>MKQYQMYVGGEWIDASNGQTEPVVSPINEEVLAYIQDADASDAERVLAVATTAQKEWAKQPARQRAEVLRKFAQLIRDNKQYLAELLVKEQGKLLKVALGEVEATSTFIEYACDWARQMDGDIVKSDNANEQIMIHKIPRGVVVAITAWNFPLALAGRKIGPALVAGNSIVVKPTSETPLATLELGYLAEQAGIPAGVLNIVTGGGRTLGNELVGHRMTNMVSMTGSTPAGQSIIRASANNMAHVQLELGGKAPFIVMEDADLEQAAAAALHSRFDNCGQVCTCNERMYVHGAVYDEFMRIFMGKVEAIKVGDPMDPASDMGPKVNANELAHMEELVAEAVDEGATVLFGGKKLEGPEFEKGFWFEPTVLTNVTQDMTIVHEESFGPILPVIKFDSFDEV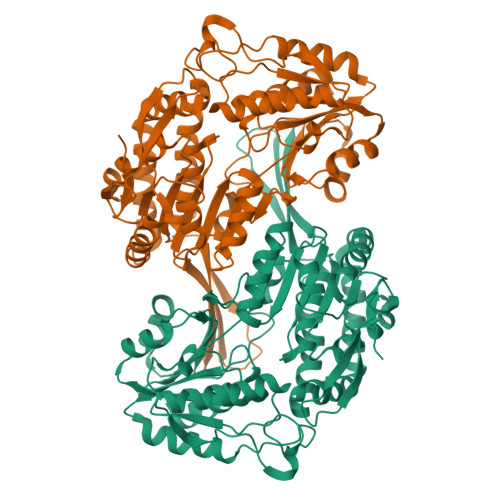IEYANDSDYGLAAMICTQNMHYINRLLTELESGEIYVNRGHGEQHQGFHNGYKLSGTGGEDGKYGFEQYLEKKTFYINYNLEHHHHHH[4x]Using X-ray crystallography, we show that the ciliopathy-associated centriolar protein CEP120 contains three C2 domains. CEP120, for example, plays a key role in the duplication, elongation, and maturation of centrioles, which in principle could impact the production of a functional basal body (Comartin et al., 2013, Lin et al., 2013, Mahjoub et al., 2010, Wu et al., 2014). All three C2 domains of CEP120 (C2A, C2B, and C2C) adopt the PLC δ1-like topology II and are structurally similar to each other (root-mean-square deviation [RMSD], 2.4–2.6 Å), with major differences found mainly in their loop length. Thus, the CEP120 C2 domains probably play a role as protein-protein interaction modules.

(but not from Homo sapiens [H.s.]) we obtained diffracting crystals that allowed a structure determination at a resolution of 1.6 Å. The structure revealed a β sandwich formed by two antiparallel four-stranded β sheets, a fold characteristic of C2 domains. In human CEP120, both the V194A JS and the A199P JATD mutations fall within the C2B domain. In our structure of C2B from Oreochromis niloticus, the equivalent residues (V195 and A200) point inward toward its hydrophobic core, suggesting that they play a structurally analogous role in stabilizing the C2B fold. The point mutations V194A and A199P, which cause Joubert syndrome (JS) and Jeune asphyxiating thoracic dystrophy (JATD), respectively, both reduce the thermostability of the second C2 domain by targeting residues that point toward its hydrophobic core. Our structures revealed neither complexed Ca2+ nor potential Ca2+-coordinating top loop residues or cationic β-grooves. Prime candidates for interaction interfaces in these domains are the regions defined by strands 3 and 4 at the edges of their β sandwich that constitute their most conserved parts. Strikingly, other structurally characterized C2 domains engage their binding partners using exactly the same interface. Both residues V194 and A199, targeted by the JS and JATD mutations, are located near this putative interface in CEP120 C2B and might disrupt its function as suggested by our in vitro experiments.

> GPHMPEKLEAILIPDQGYHQVGPADLCTDMFVLSVTVAFATKLEQLVPSTMKLSAEGSEFFFYYSLLGNDITSEPFHNLLSPDFEPERASVRIRSSKQILKAFLSQQPSLQIHLCCGNHSLGSTDVSLSALAGISTDLDNKAATVEGAFILQPPKRVKQTLPALPTDLQPTLGVAVTLRREEVALQQSVGNKE>[2x]STLKKKRTWHKHGPGQAPDVKPVQNGSQLFIKELRSRTFPSAEDVVARVPGSQLTLGYMEEHGFTEPILVPKKDGLGLAVPAPTFYVSDVENYVGPERSVDVTDVTKQKDCKMKLKEFVDYYYSTNRKRVLNVTNLEFSDTRMSSFVEPPDIVKKLSWVENYWPDDALLAKPKVTKYCLICVKDSYTDFHIDSGGASAWYHVLKGEKTFYLIRPASANISLYERWRSASNHSEMFFADQVD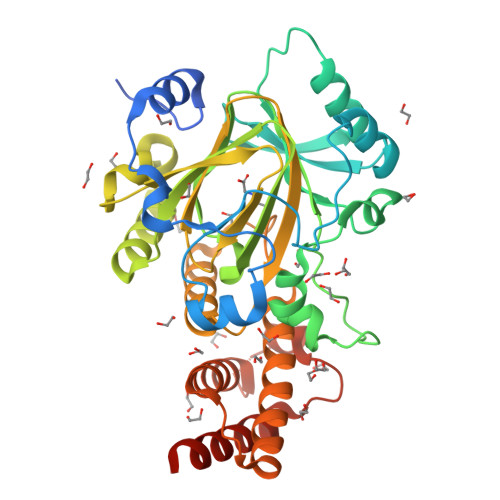KCYKCIVKQGQTLFIPSGWIYATLTPVDCLAFAGHFLHSLSVEMQMRAYEVERRLKLGSLTQFPNFETACWYMGKHLLEAFKGSHKSGKQLPPHLVQGAKILNGAFRSWTKKQALAEHEDELPEHFKPSQLIKDLAKEIRLSENASKAVRP> SLEGGVVVPVDYHLLMMFTKAEHNAPLQAKARVALSSLLRLA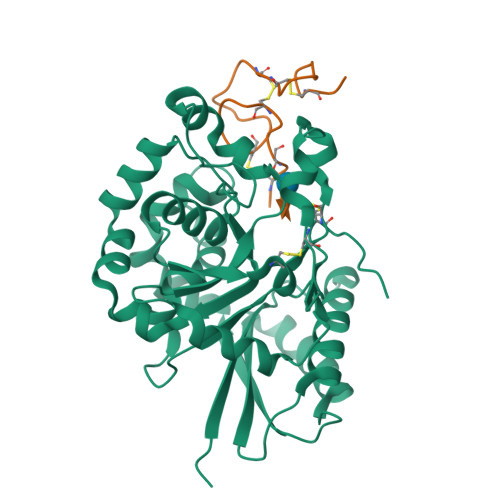KFEAHEVLNLHFVSEEASREVAKALLRELLPPAAGFKCKVIFHDVAVLTDKLFPVVEAMQKYFSAGSGTYYSDSIFFLSVAMHQIMPKEIPRIIQLDLDLKYKTNIRELFEEFDNFLPGAVIGIAREMQPVYRHTFWQFRHENPKTRVGDPPPEGLPGFNSGVMLLNLEAMRQSPLYSHLLEPSWVQQLADKYHFRGHLGDQDFFTMIGMEHPELFHVLDCTWNRQLCTWWRDHGYSDVFQAYFRCEGHVKIYHGNCNTPIPED;> MDIVDGDQCESNPCLNGGSCKDDINSYECWCPFGFEGKNCELLEHHHHHH3'-deoxy-3'-(glycylamino)adenosine | C12 H17 N7 O4 | 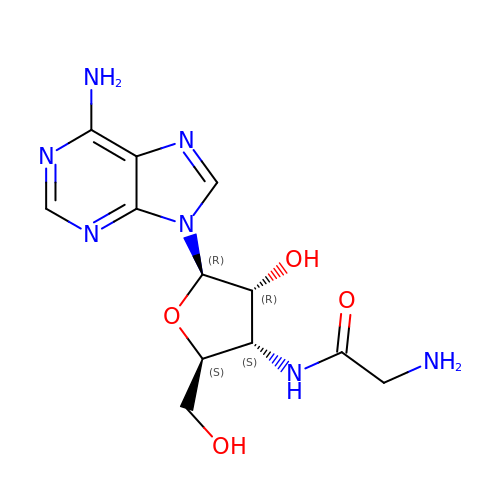XJJYXFHVLHMVGL-MUIQIWNUSA-N>[4x]GSSKSPWAN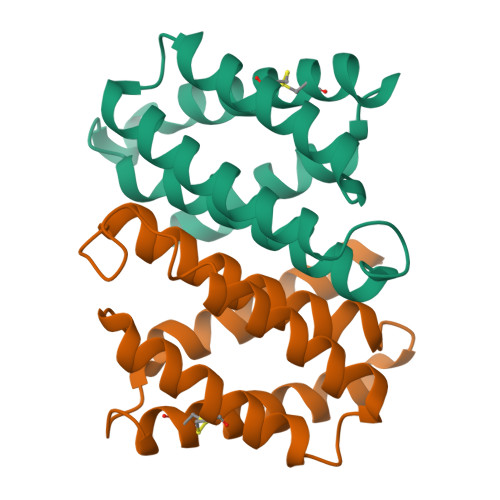PAKANAFMKCLIQKISTSPVFPQQEKEDMEEIVETMMSAFSSMSTSGGSNAAKLQAMNMAFASSMAELVIAEDADNPDSISIKTEALAKSLQQCFKSTLGSVNRHFIAEIKDLIGMFAREAAAMEEAGDEEEETY> MNNLVILPILIPFIVGTILILFAKNHSLQRVISGFTVIGMLLVAIYLAMDVYQNGISVLELGNWQAPFGIVLVADMFATMMVILASIVGVVCLFFAFQTISSEREKYYFYPFYFFLLAGVNGAFLTGDLFNLFVFFEVMLIASYILIVLGGTKYQLRESL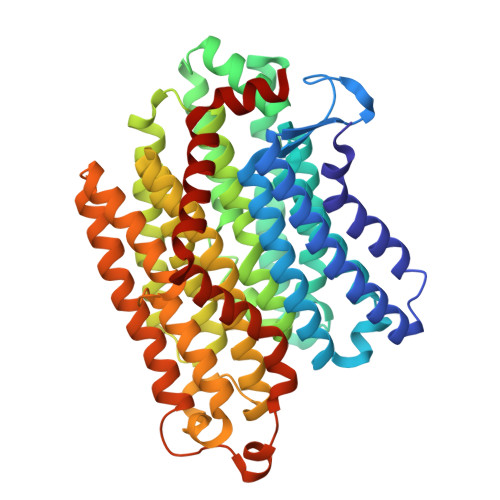KYVMINVFASILFIVGVAYIYSVTGTLNMADLAVKVGQLEQTGVLNVIAVIFLVVFAMKGGLFPLYFWLPRSYYGPPAAIAALFGGLLTKVGIYAIMRTFTLIFTHDPDFTHMLILILAGLTMFFGVLGAVSQFDFKRILSYHIISQVGYMVMGLGIYTQLAIAGAIYYIAHHIIVKAALFLFAGATQRITGTTDLKKMGGLLKTHPWLAWMFFISAISLAGIPPLSGFFSKFALILAAFLNENYIIAAVALAVGLLTLFSMMKIFIYAFWGEQKHTEQQANFKVGKLLLPIVPLVALTIILGFAAEPIFQYSLQVADQILDPTIYIESVLKE>GSHMGPVEILPFLYLGSAYHASKCEFLANLHITALLNVSRRTSEACMTHLHYKWIPVEDSHTADISSHFQEAIDFIDCVREKGGKVLVHSEAGISRSPTICMAYLMKTKQFRLKEAFDYIKQRRSMVSPNFGFMGQLLQYESEILPSTPNPQPPSCQGE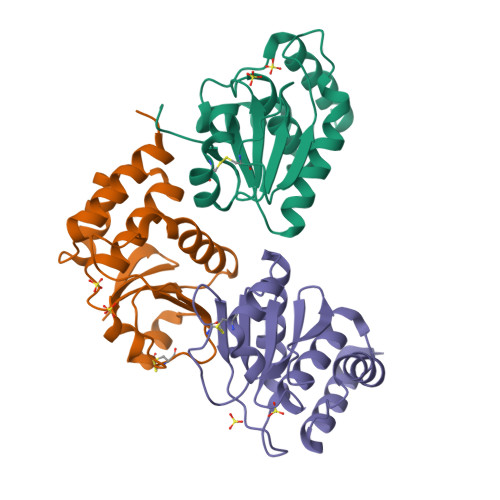AAGSSLIGHLQTLSPDMQGAYCTFPASVLAPVPTHSTVSELSRSPVATATSC[3x]> TLSILVAHDLQRVIGFENQLPWHLPNDLKHVKKLSTGHTLVMGRKTFESIGKPLPNRRNVVLTSDTSFNVEGVDVIHSIEDIYQLPGHVFIFGGQTLYEEMIDKVDDMYITVI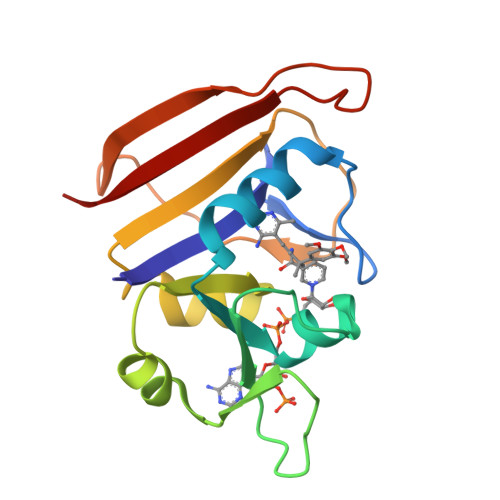EGKFRGDTFFPPYTFEDWEVASSVEGKLDEKNTIPHTFLHLIRK>[8x]MHVTQEQVMMRKMVRDFARKEIAPAAEIMEKTDEFPFQLIKKMGKHGLMGIPVPEQYGGAGADVVSYILAIHEISRISAAVGVILSVHTSVGTNPILYFGNEEQKMKYIPNLASGDHLGAFALTEPHSGSDAGSLRTTAIKKNGKYLLNGSKIFITNGGAADIYITFALTAPDQGRHGISAFIVEKNTPGFTVGKKERKLGLYGSNTTELIFDNAEVPEANLLGKEGDGFHIAMANLNVGRIGIAAQA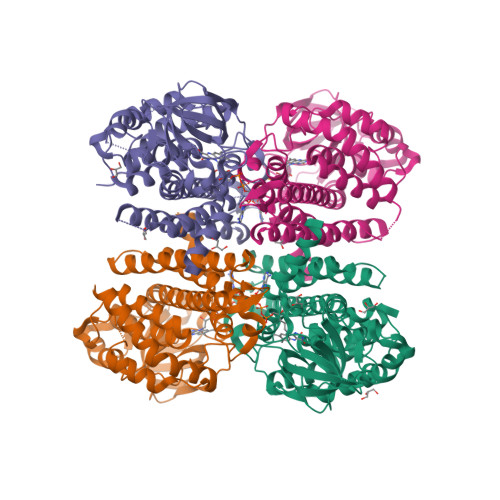LGIAEAALEHAVDYAKQRVQFGRPIAANQGISFKLADMATRAEAARHLVYHAADLHNRGLNCGKEASMAKQFASDAAVKAALDAVQIYGGYGYMKDYPVERLLRDAKVTQIYEGTNEIQRLIISKYLLGGT> MVYPQPKVLTPSRKDVLVVTPWLAPIVWEGTFNIDILNEQFRLQNTTIGLTVFAIKKYVAFLKLFLETAEKHFMVGHRVHYYVFTDQPAAVPRVTLGTGRQLSVLEVGAYKRWQD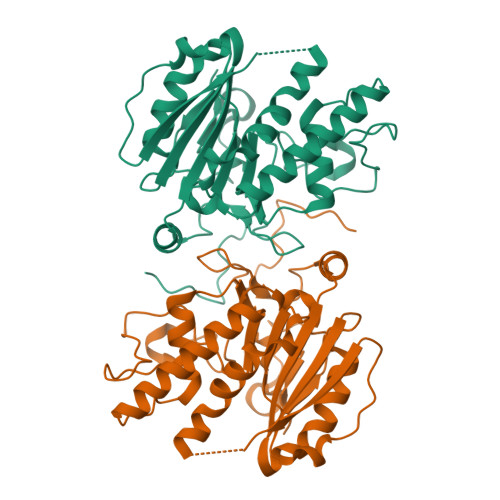VSMRRMEMISDFSERRFLSEVDYLVCVDVDMEFRDHVGVEILTPLFGTLHPSFYGSSREAFTYERRPQSQAYIPKDEGDFYYMGAFFGGSVQEVQRLTRACHQAMMVDQANGIEAVWHDESHLNKYLLRHKPTKVLSPEYLWDQQLLGWPAVLRKLRFTAVPKNHQAVRNPE>MAIPAFHPGELNVYSAPGDVADVSRALRLTGRRVMLVPTMGALHEGHLALVRAAKRVPGSVVVVS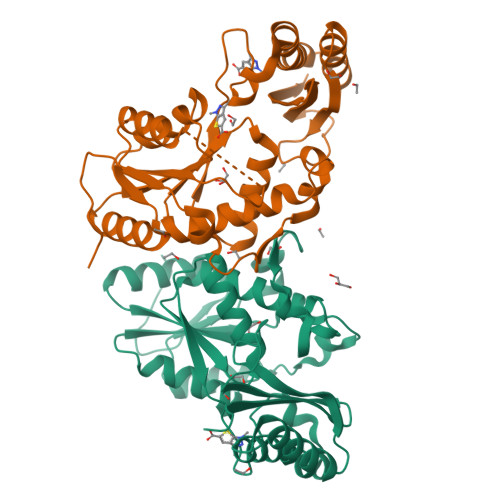IFVNPMQFGAGGDLDAYPRTPDDDLAQLRAEGVEIAFTPTTAAMYPDGLRTTVQPGPLAAELEGGPRPTHFAGVLTVVLKLLQIVRPDRVFFGEKDYQQLVLIRQLVADFNLDVAVVGVPTVREADGLAMSSRNRYLDPAQRAAAVALSAALTAAAHAATAGAQAALDAARAVLDAAPGVAVDYLELRDIGLGPMPLNGSGRLLVAARLGTTRLLDNIAIEIGTFAGTDRPDGYRA[2x]> MFRVRRLAGFIQCSPCGKMGPLKQQTRRYTPIWKSDPAVDNVAPLRDEDERRALWAEVGPISDVGSAVTAWIRFGNDPVLHTAVPTMLGGKFRNQQREKESLLPNSSSPFAYVEDYMGTNLVFGSPVHAKESAAVWATYFERRYASRLRLSRRTVANYVGLINSPEVFDDESDRPETRWSQDTFFRECAYLSEKFLKEKVSNMQQFEAALKRASPEAYLAFFDAFQQQTQTQIPLPSPSVWHYEGERRKQWAEKFISISHKAQAFFKDVLSEDVKKYQEVPGKLLQKVKPVLADVGKILVKRHERWLKGRVWTSLTEEEREAYCMKEVKRQQMQVEDGEFDPMMEDDVDDTELEEWQREHDAIMKLMNSPIDGLHFTTLELWLHTMRCEELETEHIYTSARVRAIQVAARKKLYDTTSYEEVIQAVVESIARGTLDLGAGVLRPHFNEVWCQLNYAKFGSSTITQHTTTSRRQLLFFHAGSLKDIAATATLYYATKPLSNSLDYASPYKYRRSLITLCSNYGVETAYTTQRPLLRSAANLARAEDLIHAVVTAAAQPFGERRRAATRDLHMEFQRLAVPVERVIVANPVSALLESGADPDEKPVEGEKVNMWPLGAK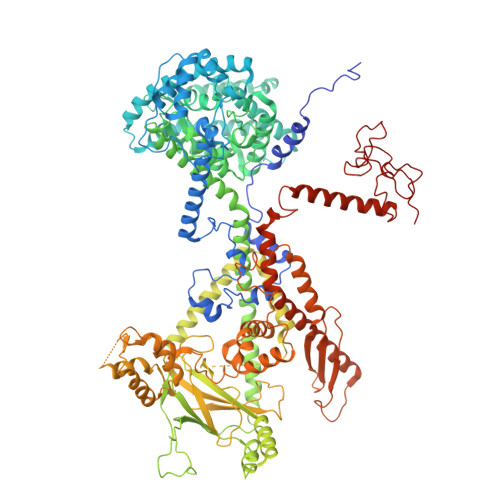RVVLYKWSAPNVEKLKAMESDAASAVSGSSLTAKRLREIQELKRRGFLEVSLWRRVTAQERKQRNEIVEAKKKQVEEVVRTVPSLAHLHQYATSLYSRIEERVAFPTETSTVTETTNMKEETNKPLEDSEWEFAVLLDDRVLLNKEESVELYLPYRDANGELLAQGEYRALVRAFDLEANPNLHPAYCSVGYSESFQVFDALPQLIAQFFRVKDATAEAAGVTHIPAADFTPFCAFLRDAGLDVPLRCEFEAGQAVTTDGDVYMDYFLQLLRGEAFHQSHAQAGLTEAQRAIEPLCRAHWVVHHPGADESEWATARRSVLDHAMQHEREWWFPNEMLDVKDVVTGSTNGLTPQMYPAAVRYGVELCTVLTAEGKFVDERGSGLSARCVVNGTGAAESVVFDTANCNGTNTTSVEDALRVAHGALRSAQDRHNTLAAFRLGPLSKQSQVLLFCGVNAYEFGGKYARTYAYAFEKAKKELEATAASGFMAPSLSHEDTERLSDQPTTSPSVDRFASTTHPEQRKAQFVPRVGPGSTPLEDPAADQKSEWS>[2x]MKLAILGAGCYRTHAASGITNFSRACEVAEMVGKPEIAMTHSTITMGAELKELAGVDEVVVADPVFDNQFTVIDDFAYEDVIEAHKEDPEKIMPQIREKVNEVAKELPKPPEGAIHFTHPEDLGFEITTDDREAVADADFIMTWFPKGDMQPDIINK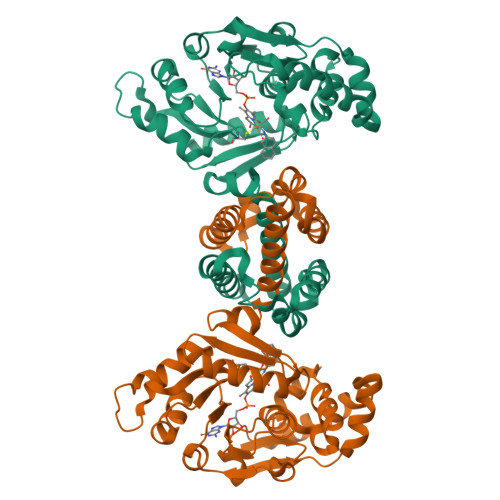FIDDIKPGAIVTHACTIPTTKFYKIFEQKHGDLVTKPETLNVTSYHPGAVPEMKGQVYIAEGYASEDAIETLFELGQKARGNAYRLPAELLGPVCDMCSALTAITYAGILSYRDSVTQVLGAPASFAQMMAKESLEQITALMEKVGIDKMEENLDPGALLGTADSMNFGASAEILPTVFEILEKRKK> MLRQTAARLNTYLTRSVATPPISVIRTGPKWWA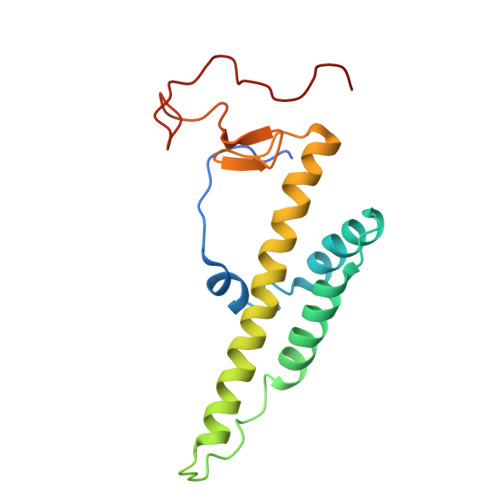EPERMVKHKVMYFTMGIDQLPLRRTAVIQKDLKRFHMCKPPPRVGDATGYKRSRGAQLTTWYRRIQYQEYHLQHLFVRHMWGLLRMYPGNTTKIQGKADDGYVGYDSVHFHRYNRSPLPFPAREIYERRK>[2x]HHHHHHSSGLVPRGSHMQSMRFMILALLVQFLPAWAIN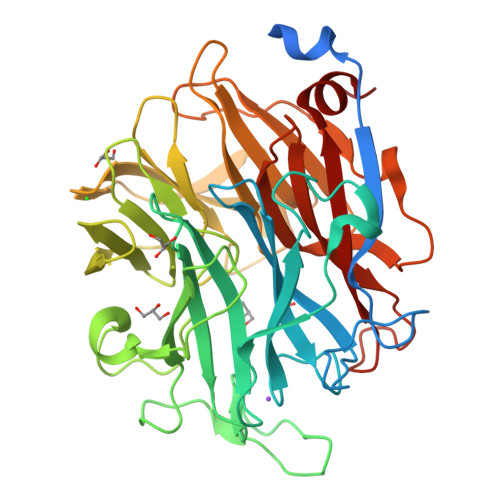DPAKSAAPYHDEFPLFRSANMASPDKLSTGIGFHSFRIPAVVRTTTGRILAFAEGRRHTNQAFGDINLVYKRTKTTANNGASPSDWEPLREVVGSGAGTWGNPTPVVDDDNTIYLFLSWNGATYSQNGKDVLPDGTVTKKIDSTWEGRRHLYLTESRDDGNTWSKPVDLTKELTPDGWAWDAVGPGNGIRLTTGELVIPAMGRNIIGRGAPGNRTWSVQRLSGAGAEGTIVQTPDGKLYRNDRPSQKGYRMVARGTLEGFGAFAPDAGLPDPACQGSVLRYNSDAPARTIFLNSASGTSRRAMRVRISYDADAKKFNYGRKLEDAKVSGAGHEGGYSSMTKTGDYKIGALVESDFFNDGTGKNSYRAIIWRRFNLSWILNGPNN> EANAPGPVPGERQLAHSKMVPIPAGVFTMGTDDPQIKQDGEAPARRVTIDAFYMDAYEVSNTEFEKFVNSTGYLTEAEKFGDSFVFEGMLS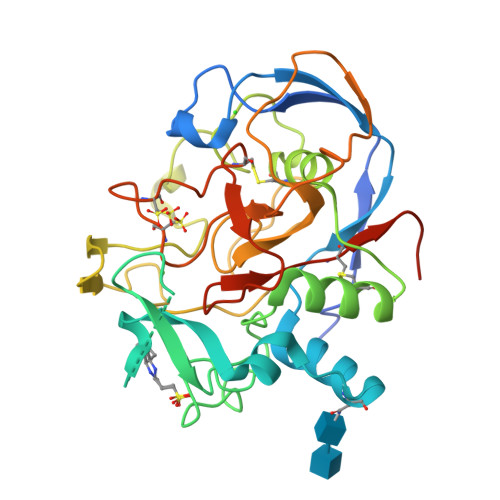EQVKTNIQQAVAAAPWWLPVKGANWRHPEGPDSTILHRPDHPVLHVSWNDAVAYCTWAGKRLPTEAEWEYSCRGGLHNRLFPWGNKLQPKGQHYANIWQGEFPVTNTGEDGFQGTAPVDAFPPNGYGLYNIVGNAWEWTSDWWTVHHSVEETLNPKGPPSGKDRVKKGGSYMCHRSYCYRYRCAARSQNTPDSSASNLGFRCAADRLPTMDRGSHHHHHH>[2x]MKSTI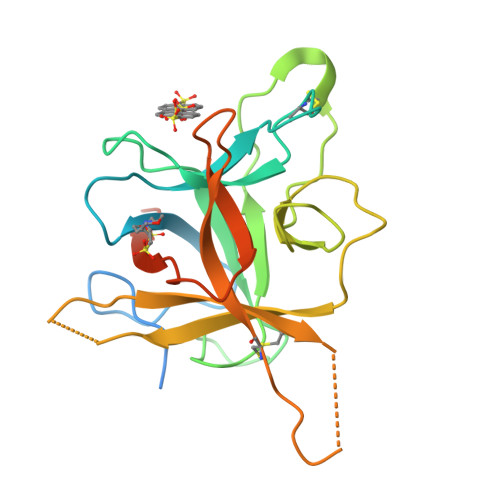FFLFLFCAFTTSYLPSAIADFVLDNEGNPLENGGTYYILSDITAFGGIRAAPTGNERCPLTVVQSRNELDKGIGTIISSPYRIRFIAEGHPLSLKFDSFAVIMLCVGIPTEWSVVEDLPEGPAVKIGENKDAMDGWFRLERVSDDEFNNYKLVFCPQQAEDDKCGDIGISIDHDDGTRRLVVSKNKPLVVQFQKLDKESLAKKNHGLSRSE> MSDKRKIQHEGIIALINYSTLCAQKCDVLKGHDDKITDTEEQCLRVCAEK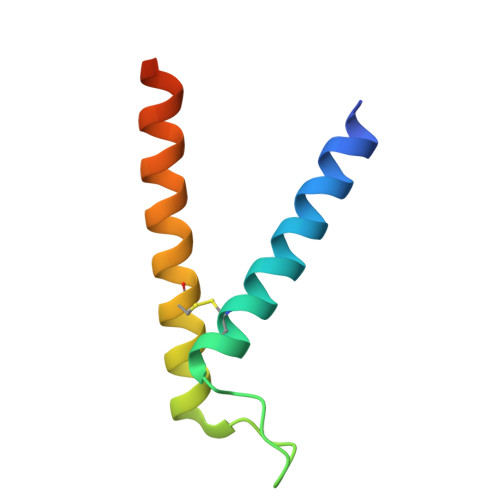IRQTFEFTNDIYLKNPNLTKPN[(1R,2R,3S,4R)-4-{[5-(1-benzyl-1H-pyrazole-3-carbonyl)pyrimidin-4-yl]amino}-2,3-dihydroxycyclopentyl]methyl 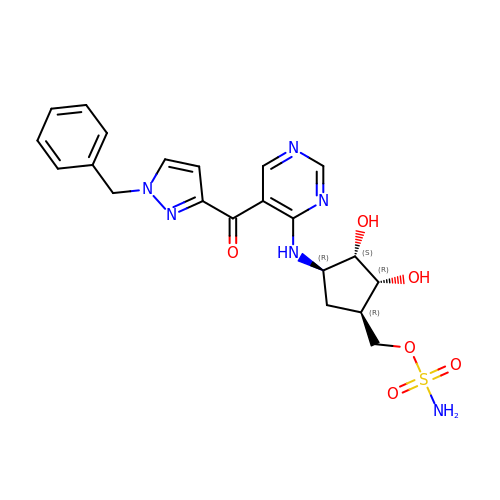sulfamate | C21 H24 N6 O6 S | AGIKMOLYLSSZIM-ZESCBINXSA-N> MSAKAISEQTGKELLYKFICTTSAIQNRFKYARVTPDTDWARLLQDHPWLLSQNLVVKPDQLIKRRGKLGLVGVNLTLDGVKSWLKPRLGQEATVGKATGFLKNFLIEPFVPHSQAEEFYVCIYATREGDYVLFHHEGGVDVGDVDAKAQKLLVGVDEKLNPEDIKKHLLVHAPEDKKEILASFISGLFNFYEDLYFTYLEINPLVVTKDGVYVLDLAAKVDATADYICKVKWGDIEFPPPFGREAYPEEAYIADLDAKSGASLKLTLLNPKGRIWTMVAGGGASVVYSDTICDLGGVNELANYGEYSGAPSEQQTYDYAKTILSLMTREKHPDGKILIIGGSIANFTNVAATFKGIVRAIRDYQGPLKEHEVTIFVRRGGPNYQEGLRVMGEVGKTTGIPIHVFGTETHMTAIVGMALGHRPIP;> GKSTTLFSRHTKAIVWGMQTRAVQ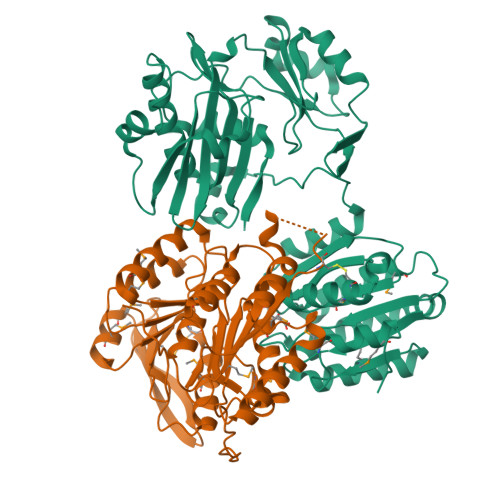GMLDFDYVCSRDEPSVAAMVYPFTGDHKQKFYWGHKEILIPVFKNMADAMRKHPEVDVLINFASLRSAYDSTMETMNYAQIRTIAIIAEGIPEALTRKLIKKADQKGVTIIGPATVGGIKPGCFKIGNTGGMLDNILASKLYRPGSVAYVSRSGGMSNELNNIISRTTDGVYEGVAIGGDRYPGSTFMDHVLRYQDTPGVKMIVVLGEIGGTEEYKICRGIKEGRLTKPIVCWCIGTCATMFSSEVQFGHAGACANQASETAVAKNQALKEAGVFVPRSFDELGEIIQSVYEDLVANGVIVPAQEVPPPT> MSDQQQPPVYKIALGIEYDGSKYYGWQRQNEVRSVQEKLEKALSQVANEPITVFCAGRTDAGVHGTGQVVHFETTALRKDAAWTLGVNANLPGDIAVRWVKTVPDDFHARFSATARRYRYIIYNHR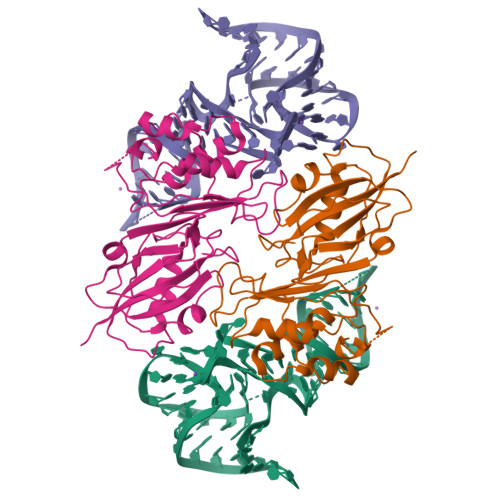LRPAVLSKGVTHFYEPLDAERMHRAAQCLLGENDFTSFRAVQCQSRTPWRNVMHINVTRHGPYVVVDIKANAFVHHMVRNIVGSLMEVGAHNQPESWIAELLAAKDRTLAAATAKAEGLYLVAVDYPDRYDLPKPPMGPLFLAD>[2x]GPLGSMDGTAAEPRPGAGSLQHAQPPPQPRKKRPEDFKFGKILGEGSFSTVVLARELATSREYAIKILEKRHIIKENKVPYVTRERDVMSRLDHPFFVKLYFTFQDDEKLYFGLSYAKNGELLKYIRKIGSFDETCTRFYTAEIVSALEYLHGKGIIHRDLKPENILLNEDMHIQITDFGTAKVLSPESKQARANSFVGTAQYVSPELLTEKSACKSSDLWALGCIIYQLVAGLPPFRAGNEYLIFQK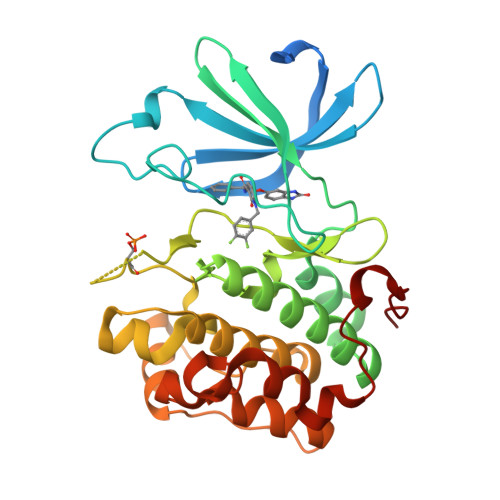IIKLEYDFPAAFFPKARDLVEKLLVLDATKRLGCEEMEGYGPLKAHPFFESVTWENLHQQTPPKLT>MTATDNARQVTIIGAGLAGTLVARLLARNGWQVNLFERRPDPRIETGARGRSINLALAERGAHALRLAGLEREVLAEAVMMRGRMVHVPGTPPNLQPYGRDDSEVIWSINRDRLNRILLDGAEAAGASIHFNLGLDSVDFARQRLTLSNVSGERLEKRFHLLIGADGCNSAVRQAMASVVDLGEHLETQPHGYKELQITPEASAQFNLEPNALHIWPHGDYMCIALPNLDRSFTVTLFLHHQSPAAQPASPSFAQLVDGHAARRFFQRQFPDLSPMLDSLEQDFEHHPTGKLATLRLTTWHVGGQAVLLGDAAHPMVPFHGQGMNCALEDAVALAEHLQSAADNASALAAFTAQRQPDALAIQAMALENYVEMSSKVASPTYLLERELGQIMAQRQPTRFIPRYSMVTFSRLPYAQAMARGQIQEQLLKFAVANHSDLTSINLDAVEHEVTRCLPPLSHLS[2x]

Kynurenine-3-monooxygenase (KMO) is a class A flavoprotein monooxygenase (FPMO) which catalyses the hydroxylation of L-kynurenine (L-Kyn) to 3-hydroxykynurenine (3-HK), using NADPH as a co-substrate. It lies at a key branch point of the kynurenine pathway and its expression is largely restricted to the liver, kidney, some monocytic cells, and to a lesser extent in the microglia within the brain. We therefore turned our attention to the homologous bacterial P. fluorescens enzyme, Pf-KMO, which shares 34% sequence identity with the human enzyme, but lacks the transmembrane region and had been previously extensively characterized by Crozier-Reabe et al.. The KMO monomer consists of three domains: the α+β FAD-binding domain, an α+β domain containing a six-stranded, mostly antiparallel, β-sheet and a C-terminal four-helix bundle domain.

Unexpectedly, a jump in affinity occurred when alkoxyl-linked pyridyl groups such as those present in GSK891(B1) and GSK775(B2) were added. A structure of GSK775(B2) in Pf-KMO confirmed that it binds within the substrate site, with the oxazolidinone core overlapping almost exactly with that in series A compounds. However, the pendant pyridyl group does not reside in the water filled pocket as modelled in Fig. 4e,f. Instead, it π-stacks against a flavin group that is now tilted away from the substrate site in an orientation not previously observed in KMO, or any other FPMOs we have found. In addition to the face to face π interaction with FAD the pyridine also makes edge to face π interactions with Y193 and F238. Flavin movement creates a new solvent channel that opens the active site to the protein surface, the pyridine nitrogen of GSK775(B2) H-bonds with an extended water network within this opening. R111 needs to move in concert with this flavin tilt, but few other protein changes are necessary to accommodate this movement. Taken together these data suggest a differentiated kinetic profile for GSK775(B2) and GSK428(A2), with GSK775(B2) showing slow onset of inhibition and slow dissociation, in contrast to the rapid kinetics of GSK428(A2). The apparently non-competitive behaviour of GSK775(B2) can be rationalized by the unexpected slow dissociation of the prebound inhibitor relative to the timescale of the initial competition assay (∼2 h half life for the KMO-GSK775(B2) complex). Crystallographic complexes of our extended oxazolidinone inhibitor series (B) rationalize their unexpectedly high potency, by demonstrating that they bind with this intriguing variation of the flavin position.> MSEDIQPMETVGATDTGAGAQVDPRTGGQAAGGSGGMGAGGSANDGRQDIFSGAPQPNQHHTLVYGKSYHFTITNGLPEFRHLATTN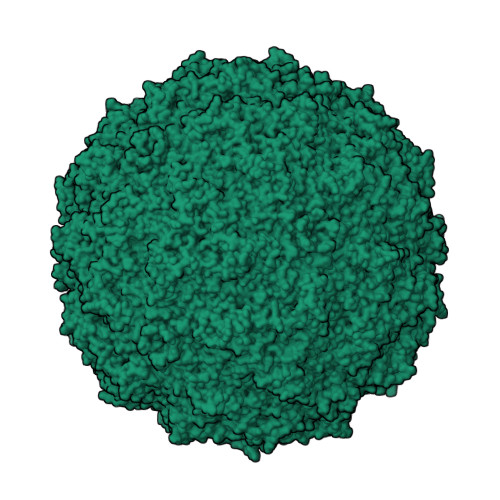SGYYAQQRFKHIHGIPWERLLMYVSEGELLRMFRDYTSLKVEEVVCEVYSLGVRLPFVTSATTSSVANANAQYPIGCFHFDEAYETNYGINNVADIINKALGTEWKNATRPTAAVTTAWSEQFPNISASSTSRDINNPVIVDYSLPYFENNVPKDVGIYDYVDIKNGTTAYGKCWEKRFKPTNGLLYAESTLKGNVVTPLAAQPTNIMTPIPGLENGYFMSNDQIRERRDLTTSVPPVALTATKLNQSASNNLNAFVDYMGYNYFGEQKCAPQSMPKFMIGFVNIRNEDNSLLNAKWDILIKTRIRLTGLQSTREWVARTDRIPPQYFTSQYTQFRYPNINETPLLRSLGTFKLPTKRPGMDSRIAAGRAAETTQDEFIDAQKKLRHKSALLPIIEKPVTRSSKLNK>[2x]MMYKEPFGVKVDFETGIIEGAKKSVRR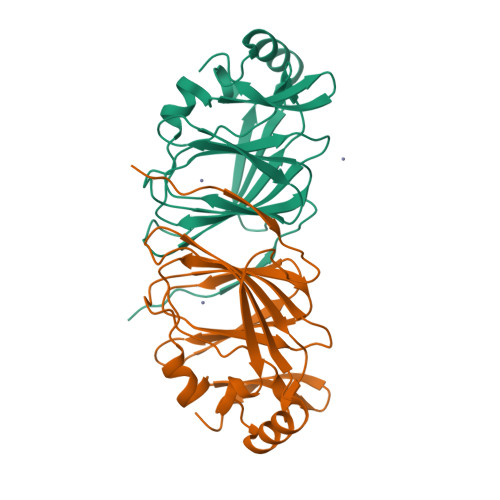LSDMEGYFVDERAWKELVEKEDPVVYEVYAVEQEEKEGDLNFATTVLYPGKVGKEFFFTKGHFHAKLDRAEVYVALKGKGGMLLQTPEGDAKWISMEPGTVVYVPPYWAHRTVNIGDEPFIFLAIYPADAGHDYGTIAEKGFSKIVIEENGEVKVVDNPRW ExbB and ExbD are cytoplasmic membrane proteins that associate with TonB to convey the energy of the proton-motive force to outer membrane receptors in Gram-negative bacteria for iron uptake. The opportunistic pathogen Serratia marcescens (Sm) possesses both TonB and a heme-specific TonB paralog, HasB. ExbBSm has a long periplasmic extension absent in other bacteria such as E. coli (Ec). We purified ExbBSm alone and ExbBDSm and determined their structures by single-particle cryo-EM at 3.1 and 3.96 Å resolution, respectively.

The 3D class average model clearly showed a pentameric structure. It was refined and polished to obtain a resolution of 3.1 Å using the Fourier shell correlation (FSC) gold-standard criterion at 0.143. The periplasmic N-terminal extension did not yield any visible density, precluding its structure determination. At the C-terminus of each monomer, however, density was clearly defined, allowing structure determination for an additional 10 residues in a helical conformation up to the last one (helix α8 finishing with Gly 283) before the His-tag that is present but disordered. The cryo-EM density of ExbBSm shows vents located at the interface of adjacent monomers and at the height of the cytoplasmic junction with the inner membrane leaflet. These vents may allow solvent or ion passage. Additional density was also clearly observed on the external surface, and we attributed it to the phospholipids present in the preparation. Each ExbB monomer appears to be associated with the equivalent of two PG molecules, located at the inner leaflet of the cytoplasmic membrane. However, we were able to model only one PG molecule per monomer with confidence.

>[5x]APAANPAVTESVAPTTAPAPAAAAPESITPVNPAPTIQPPETRGMDLSIWGMYQHADAVVKAVMIGLVLASIVTWTILFAKGSELLRAKRRLRREQLALAEARSLDEASELAQNFSPESVSAVLLNDAQNELELSAESNDNNGIKERTGFRLERRVAAYSRNMGRGNGFLATIGAISPFVGLFGTVWGIMNSFIGIAHSQTTNLAVVAPGIAEALLATAMGLVAAIPAVVIYNIFARVISGHRAQVGDVAAQVLLLQGRDLDLAATAEAKRSQHAHQLRAGHHHHHH> ASDYKDDDDKGALEVLFQGPSSPMAGNLVSWACKLCRSPEGFGPISFYGDFTQCFIDGVILNLSAIFMITFGIRDLVNLCKKKHSGIKYRRNWIIVSRMALVLLEIAFVSLASLNISKEEAENFTIVSQYASTMLSLFVALALHWIEYDRSVVANTVLLFYWLFETFGNFAKLINILIRHTYEGIWYSGQTGFILTLFQVITCASILLLEALPKKPLMPHQHIHQTLTRRKPNPYDSANIFSRITFSWMSGLMKTGYEKYLVEADLYKLPRNFSSEELSQKLEKNWENELKQKSNPSLSWAICRTFGSKMLLAAFFKAIHDVLAFTQPQLLRILIKFVTDYNSERQDDHSSLQGFENNHPQKLPIVRGFLIAFAMFLVGFTQTSVLHQYFLNVFNTGMYIKSALTALIYQKSLVLSNEASGLSSTGDIVNLMSVDVQKLQDLTQWLNLIWSGPFQIIICLYSLYKLLGNSMWVGVIILVIMMPLNSFLMRIQKKLQKSQMKYKDERTRVISEILNNIKSLKLYAWEKPYREKLEEVRNNKELKNLTKLGCYMAVTSFQFNIVPFLVSCCTFAVFVYTEDRALTTDLVFPALTLFNLLSFPLMIIPMVLNSFIEASVSIGRLFTFFTNEELQPDSVQRLPKVKNIGDVAINIGDDATFLWQRKPEYKVALKNINFQAKKGNLTCIVGKVGSGKTALLSCMLGDLFRVKGFATVHGSVAYVSQVPWIMNGTVKENILFGHRYDAEFYEKTIKACALTIDLAILMDGDKTLVGEKGISLSGGQKARLSLARAVYARADTYLLDDPLAAVDEHVARHLIEHVLGPNGLLHTKTKVLATNKVSALSIADSIALLDNGEITQQGTYDEITKDADSPLWKLLNNYGKKNNGKSNEFGDSSESSVRESSIPVEGELEQLQKLNDLDFGNSDAISLRRASDATLGSIDFGDDENIAKREHREQGKVKWNIYLEYAKACNPKSVCVFILFIVISMFLSVMGNVWLKHWSEVNSRYGSNPNAARYLAIYFALGIGSALATLIQTIVLWVFCTIHASKYLHNLMTNSVLRAPMTFFETTPIGRILNRFSNDIYKVDALLGRTFSQFFVNAVKVTFTITVICATTWQFIFIIIPLSVFYIYYQQYYLRTSRELRRLDSITRSPIYSHFQETLGGLATVRGYSQQKRFSHINQCRIDNNMSAFYPSINANRWLAYRLELIGSIIILGAATLSVFRLKQGTLTAGMVGLSLSYALQITQTLNWIVRMTVEVETNIVSVERIKEYADLKSEAPLIVEGHRPPKEWPSQGDIKFNNYSTRYRPELDLVLKHINIHIKPNEKVGIVGRTGAGKSSLTLALFRMIEASEGNIVIDNIAINEIGLYDLRHKLSIIPQDSQVFEGTVRENIDPINQYTDEAIWRALELSHLKEHVLSMSNDGLDAQLTEGGGNLSVGQRQLLCLARAMLVPSKILVLDQATAAVDVETDKVVQETIRTAFKDRTILTIAHRLNTIMDSDRIIVLDNGKVAEFDSPGQLLSDNKSLFYSLCMEAGLVNENGLVPRGSSAHHHHHHHHHHGA

Yeast Cadmium Factor 1 (Ycf1) sequesters heavy metals and glutathione into the vacuole to counter cell stress. Ycf1 belongs to the ATP binding cassette C-subfamily (ABCC) of transporters, many of which are regulated by phosphorylation on intrinsically-disordered domains. In asymmetric ABC transporters, like Ycf1, only one of two NBDs (NBD2) is capable of efficient ATP hydrolysis. Biochemical data further show R-domain phosphorylation reorganizes the Ycf1 architecture and is required for maximal ATPase activity.

In this study, we have used cryo-EM to determine the 3.4 and 4.0 Å resolution structures of endogenously phosphorylated Saccharomyces cerevisiae Ycf1 in two inward-facing conformations: wide (IFwide) and narrow (IFnarrow). We designated the state in which the NBDs are further apart as IFwide and the state in which the NBDs are closer as IFnarrow. The R-domain encircles NBD1 in both IFwide and IFnarrow and is stabilized by extensive contacts along a basic groove of the NBD1 perimeter, intracellular loop 4, and the Lasso motif. The electrostatic interactions are supported by a substantial burying of hydrophobic surfaces at 3 sites (site 1: I621 - L802 - I902 - I904; site 2: F917 - I1123 - L1120; and site 3: L912 - I915 - I1154). These interactions are poised to provide a large thermodynamic driving force of R-domain binding and stabilize the R-domain/NBD1 interface, burying ~1550 Å2 and ~1283 Å2 of surface area along the entire R-domain in IFnarrow and IFwide, respectively (~546 Å2 (IFnarrow) and ~425 Å2 (IFwide) specifically between NBD1 and the R-domain). Instead, a rearrangement within the R-domain correlates with overall movements in the structure, including a change in angle between residues G913, G918, and G932 of the R-domain from 130° (IFwide) to ~137° (IFnarrow). In contrast to the interaction sites themselves, the major structural consequences of the IFwide to IFnarrow transition are induced at the ATP-binding sites. These sites not only move closer in IFnarrow but also rotate to occlude the non-functional ATP-binding site in NBD1. Notably, the second site in NBD2 (active) is open for ATP binding. Overall, these architectural changes resemble changes in substrate-bound and substrate-free states of the Ycf1 homolog MRP1. These movements support a model where R-domain phosphorylation helps stabilize NBD1 to recruit other domains into a conformation (IFnarrow) suitable for ATP binding and initiation of transport. The tighter assembly in IFnarrow compared to IFwide may reflect the end result of the transition initiated by R-domain phosphorylation that leave key components of the transport cycle (ie NBDs, X-loop, GRD motif) engaged.>CCAGGCCTG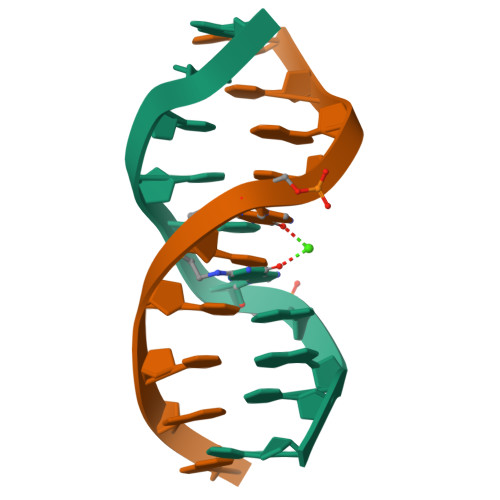G[4x]> GTSMETFDPTELPELLKLYYRRLFPYSQYYRWLNYGGVIKNYFQHRE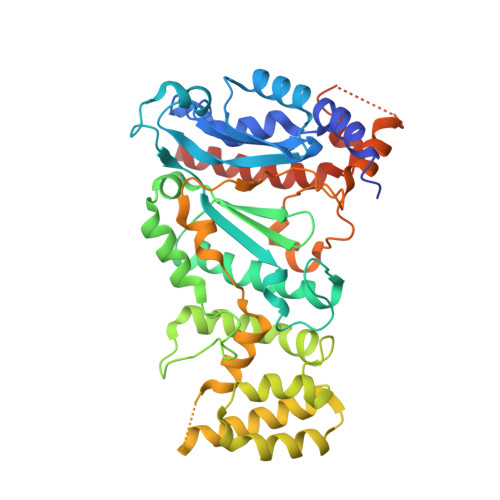FSFTLKDDIYIRYQSFNNQSDLEKEMQAANPYKIDIGAVYSHRPNQHNTVKLGAFQAQEKELVFDIDMTDYDDVRRCCSSADICPKCWTLMTMAIRIIDRALKEDFGFKHRLWVYSGRRGVHCWVCDESVRKLSSAVRSGIVEYLSLVKGGQDVKKKVHLSEKIHPFIRKSINIIKKYFEEYALVNQDILENKESWDKILALVPETIHDELQQSFQKSHNSLQRWEHLKKVASRYQNNIKNDKYGPWLEWEIMLQYCFPRLDINVSKGINHLLKSPFSVHPKTGRISVPIDLQKVDQFDPFTVPTISFICRELDAISTNEEEKEENEAESDVKHRTRDYKKTSLAPYVKVFEHFLENLDKSRKGELLKKSDLQKDF> MPTKAVTFYEDINYGGAHVHLQPGNYTLSQLNTAKIPNDWMTSLKVPSGWTVDVYENDNFTGTKWTYTSDTP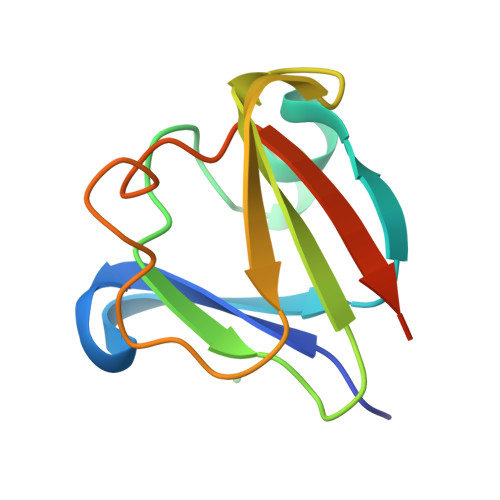WVGNDANDKMTSVKIYSTTNTGGDT> SDTAPAGFQLERVVILSRHGVRAPTKMTQTMRDVTPHQWPEWPVKLGYITPRGEHLISLMGGFYRERFQQQGLLPKDNCPTPDAVYVWADVDQRTRKTGEAFLAGLAPQCDLAIHHQQNTQQADPLFHPVKAGICSMDKSQVHAAVEKQAGTPIETLNQRYQASLALMSSVLDFPKSPYCQQHNISKLCDFSQAMPSRLAINDDGNKVALEGAV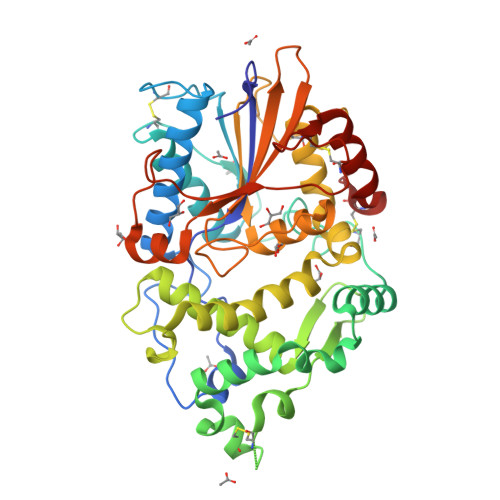GLASTLAEIFLLEHAQGMPKVAWGNIHTEQQWNSLLKLHNAQFDLMSRTPYIAKHNGTPLLQTIAHALGSNITSRPLPDISPDNKILFIAGHDTNIANISGMLGMTWTLPGQPDNTPPGGALVFERWVDNAGKPYVSVNMVYQTLAQLHDQAPLTLQHPAGSVRLNIPGCSDQTPDGYCPLSTFSRLVSHSVEPACQLP>MKTISNLTEHGEAHDHAGTPAPALPSRDVLETAGELLRALAAPLRIAIVLQLKQSQRCVHELVDA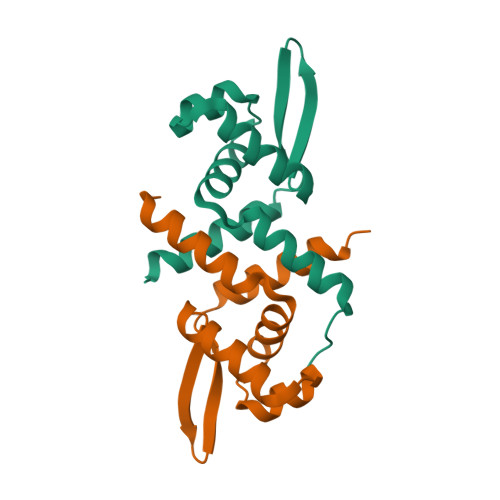LDVPQPLVSQHLRILKQAGVVSSERAGREVLYRLVDHHLAHIVVDAIAHASEDRR[2x]> NDHINLKVAGQDGSVVQFKIKRHTPLSKLMKA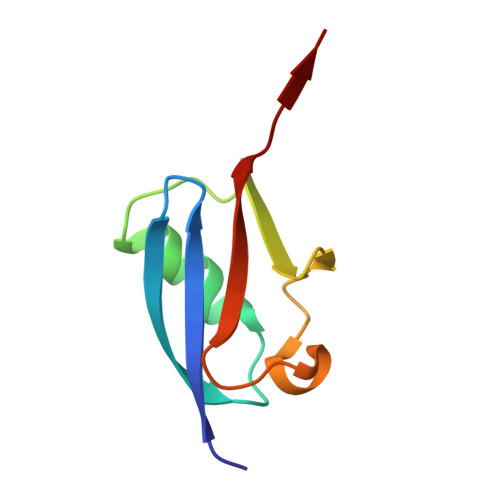YCERQGLSMRQIRFRFDGQPINETDTPAQLEMEDEDTIDVFQQQTGG>[2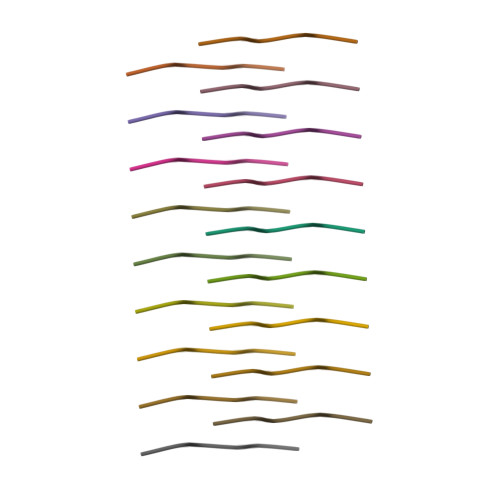x]NTVTFN> QQDLAPQQRAAPQQKRSSPS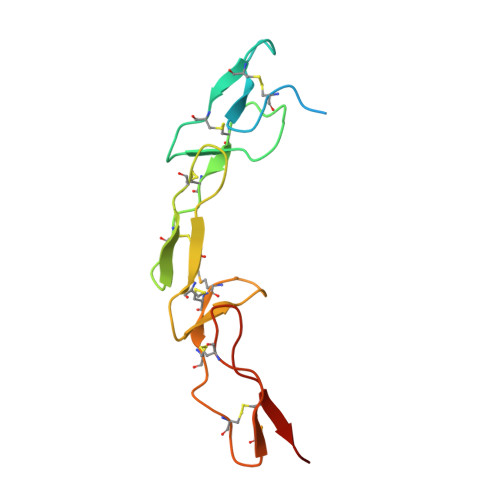EGLCPPGHHISEDGRDCISCKYGQDYSTHWNDLLFCLRCTRCDSGEVELSPCTTTRNTVCQCEEGTFREEDSPEMCRKCRTGCPRGMVKVGDCTPWSDIECVHKESG>MGSITENTSWNKEFSAEAVNGVFVLCKSSSKSCATNDLARASKEYLPASTFKIPNAIIGLETGVIKNEHQVFKWDGKPRAMKQWERDLTLRGAIQVSAVPVFQQIAREVGEVRMQKYLKKFSYGNQNISGGIDKFWLEGQLRISAVNQVEFLESLYLNKLSASKENQLIVKEALVTEA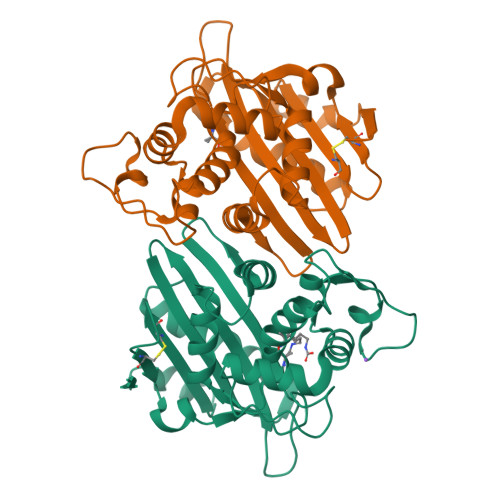APEYLVHSKTGFSGVGTESNPGVAWWVGWVEKETEVYFFAFNMDIDNESKLPLRKSIPTKIMESEGIIG[2x]>[8x]MAVESSQIPEKTVEQIFDERYPLDKWKDSNYSILDKFSMRGRKGFVTGAAGGLGRNAAAALAQAGADVALVDLPSQEDKLTELAKDMSERFGTNVIALTCDVTDTVQVAELKTQLVEQLGTVDFAFLNAGVNVPGDDQDATEEVWTRTININ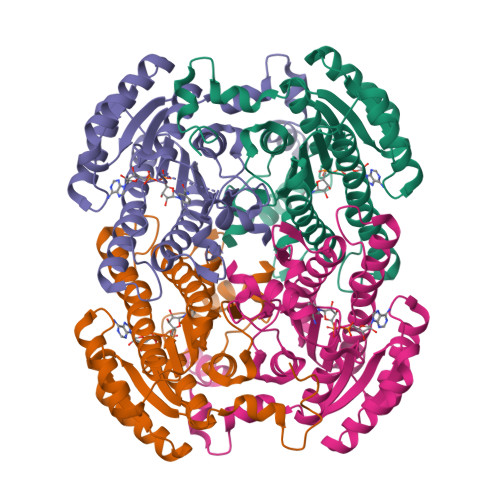LNGTYRTGRIAHEIMREHGHGGSLIFTAALSGHNANYMMGSPTPVNAYGATKAAIMEHSRYLAAALAKDGIRSNTISPGYVWSGIFNGRIDMPGHDAMLEVVPMHRFGTNDEIASTVLFLASDASSYVTGTDIRVDGGYSVF> SSYSYDAPSDFINFSSLDDEGDTQNIDSWFELKANL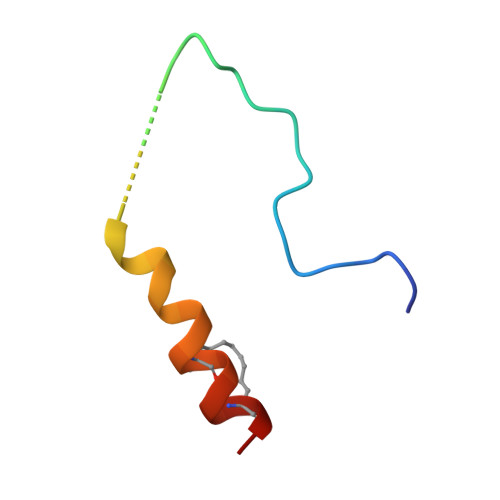ENX>[10x]MKYFLDSAILEEIRYAYENWAIDGVTTNPRHIMNSGKPFLTVLDEFASEFKGVENFPISVEINPHLDNAKDMVEEGTKIAKLSSNFVIKI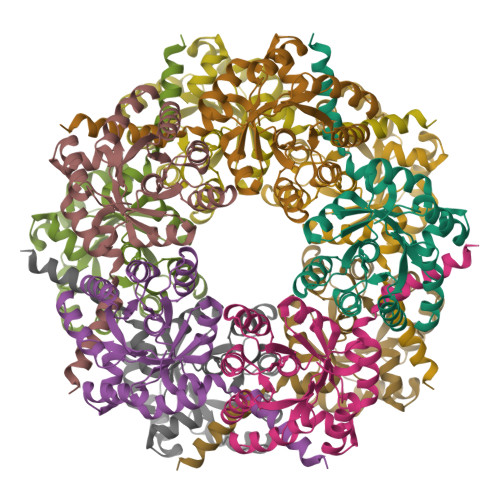PCTEPGLIAAKEFEKQGISTNVTLVFSPSQALQPARIGAKFVSPFVGWKENSGDDTTYIQDIVNIYKNYNYNTEIIVAALRNGKQIVDAAKAGAHIVTCGFDVYKESFQHAFTDYGLNKFRNAWDNTV>[24x]MSQSGEDLHSPTY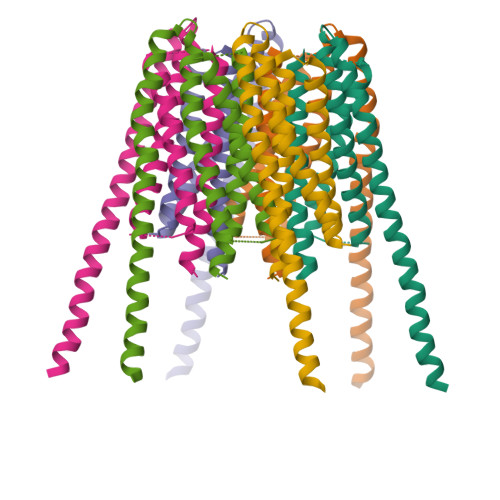LSWRKLQLSRAKLKASSWTSALLSGFAMVAMVEVQLDHDTNVPPGMLIAFAICTTLLVAVHMLALMISTCILPNIETVSNLHSISLVHESPHERLHWYIETAWAFSTLLGLILFLLEIAILCWVKFYDLSPPAAWSATVVLIPVMIIFMAFAIHFYRSLVSHKYEVTVSGIRELEMLKEQMEQDHLEHHNNIRNNGEGEEF> MAGLPNSSNALQQWHHLFEAEGTKRSPQAQQHLQQLLRTGLPTRKHENWKYTPLEGLINSQFVSIAGEISPQQRDALALTLDSVRLVFVDGRYVPALSDATEGSGYEVSINDDRQGLPDAIQAEVFLHLTESLAQSVTHIAVKRGQRPAKPLLLMHITQGVAGEEVNTAHYRHHLDLAEGAEATVIEHFVSLNDARHFTGARFTINVAANAHLQHIKLAFENPLSHHFAHNDLLLAEDATAFSHSFLLGGAVLRHNTSTQLNGENSTLRINSLAMPV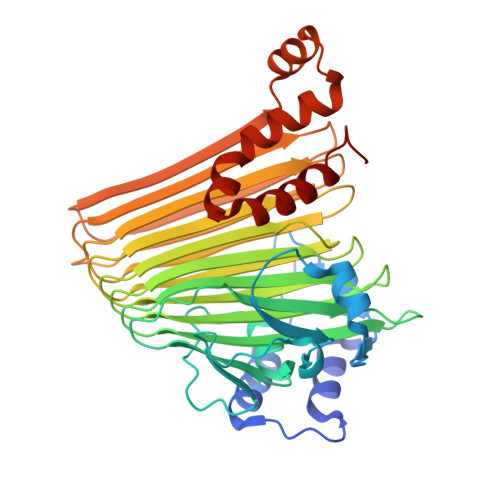KNEVCDTRTWLEHNKGFCNSRQLHKTIVSDKGRAVFNGLINVAQHAIKTDGQMTNNNLLMGKLAEVDTKPQLEIYADDVKCSHGATVGRIDDEQIFYLRSRGINQQDAQQMIIYAFAAELTEALRDEGLKQQVLARIGQRLPGGAR> PISPIETVPVKLKPGMDGPKVKQWPLTEEKIKALVEICTEMEKEGKISKIGPENPYNTPVFAIKKKDSTK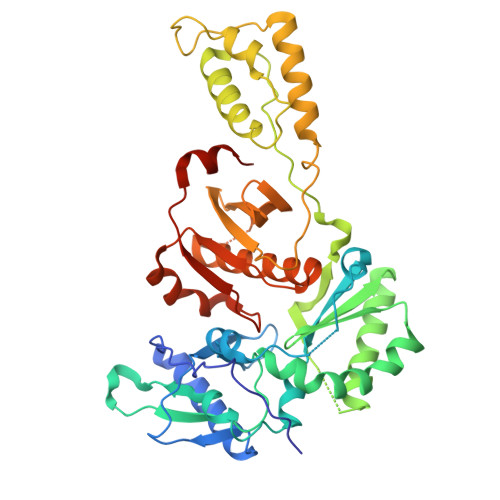WRKLVDFRELNKRTQDFWEVQLGIPHPAGLKKKKSVTVLDVGDAYFSVPLDEDFRKYTAFTIPSINNETPGIRYQYNVLPQGWKGSPAIFQSSMTKILEPFRKQNPDIVIYQYVDDLYVGSDLEIGQHRTKIEELRQHLLRWGLTTPDKKHQKEPPFLWMGYELHPDKWTVQPIVLPEKDSWTVNDIQKLVGKLNWASQIYPGIKVRQLCKLLRGTKALTEVIPLTEEAELELAENREILKEPVHGVYYDPSKDLIAEIQKQGQGQWTYQIYQEPFKNLKTGKYARMRGAHTNDVKQLTEAVQKITTESIVIWGKTPKFKLPIQKETWETWWTEYWQATWIPEWEFVNTPPLVKLWYQLEKEPIVGAETF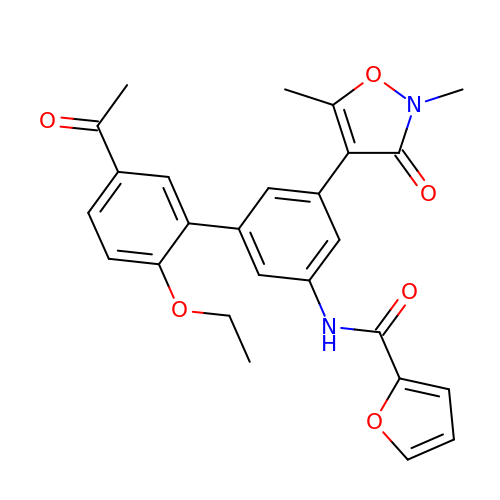~{N}-[3-(2,5-dimethyl-3-oxidanylidene-1,2-oxazol-4-yl)-5-(5-ethanoyl-2-ethoxy-phenyl)phenyl]furan-2-carboxamide | C26 H24 N2 O6 | STAVPWADWLEVHH-UHFFFAOYSA-N> GHMAQRHLDPTDPLAGPSPTGDTLAGYLRAQATEFLRALRLHRETGSGANGAEGPVEAARALRRSARRISATLHTFQSLLDTDWCEGMRPELAWVSGTLAMEHAYTARLERLLNALHRLSGSTALPSQTADSAAGGRAAGAAPVPRTAAPRDAGLRTPPTSTTERGNLTVGAAKAGALLDRQLTLARTRAHSTALQAMGSSRFHAIADKVAVLASEVPLTPAAATADLRPLATAAKDRLT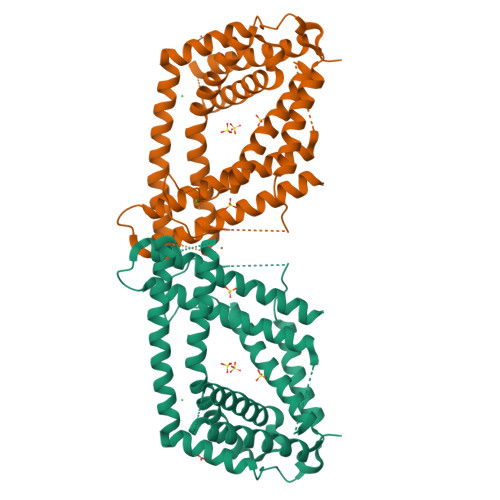DAVAALPLITAGHPYNAAALIHGLSPDTVPHPQDAPWHQVRLLLRLHRYAREAVSGPKGNAVVDLRLLSAGQALNRHRDASEAAAAAAQAARTPRIAPATAYALGVLHADQRHEVEAARFAFQQAWQKEAEAVSTR> GRTCPKPDDLPFSTVVPLKTFYEPGEEITYSCKPGYVSRGGMRKFICPLTGLWPINTLKCTPRVCPFAGILENGAVRYTTFEYPNTISFSCNTGFYLNGADSAKCTEEGKWSPELPVCAPIICPPPSIPTFATLRVYKPSAGNNSLYRDTAVFECLPQHAMFGNDTITCTTHGNWTKLPECREVKCPFPSRPDNGFVNYPAKPTLYYKDKATFGCHDGYSLDGPEEIECTKLGNWSAMPS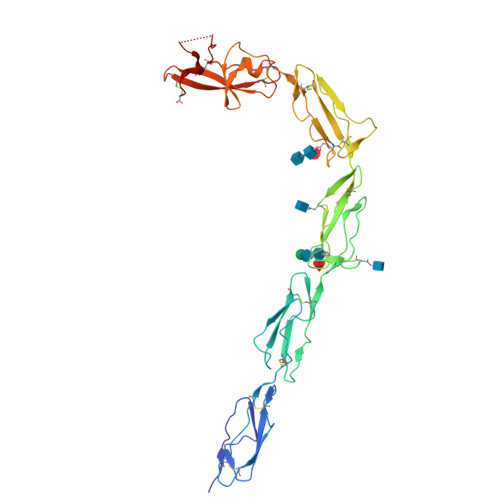CKASCKVPVKKATVVYQGERVKIQEKFKNGMLHGDKVSFFCKNKEKKCSYTEDAQCIDGTIEVPKCFKEHSSLAFWKTDASDVKPC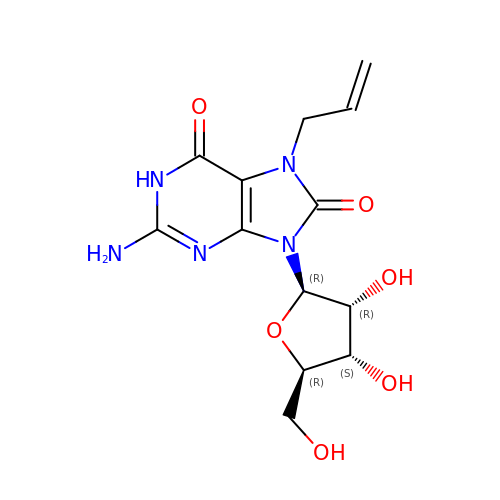2-azanyl-9-[(2~{R},3~{R},4~{S},5~{R})-5-(hydroxymethyl)-3,4-bis(oxidanyl)oxolan-2-yl]-7-prop-2-enyl-1~{H}-purine-6,8-dione | C13 H17 N5 O6 | VDCRFBBZFHHYGT-IOSLPCCCSA-N>[6x]MAPLRKTYV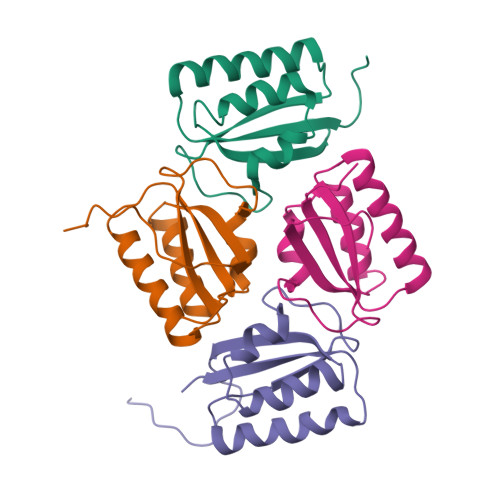LKLYVAGNTPNSVRALKTLNNILEKEFKGVYALKVIDVLKNPQLAEEDKILATPTLAKVLPPPVRRIIGDLSNREKVLIGLDLLYEEIGDQAEDDLGLE> GSAEDKSKRDSIGLNAKEGQTNNGFVQNEDILETDLDPSSPAAGPQHNTVDILGPGEPDVKDVRPYAGMPKEVLFQFSGQARYRIPREVLFWLTVASVLLLIAATIAIIAISPKCLDWWQAGPMYQIYPRSFRDSNKDGDGDLKGIQDKLDYITTLNIKTVWITSFYKSSLKDFRHAVEDFQEIDPIFGTMKDFENLVAAIHDKGLKLIIDFIPNHTSDKHAWFQWSRNRTGKYTDYYIWHDCNYENGTTIPPNNWLSVYGNSSWHFDEVRKQCYFHQFMKEQPDLNFRNPDVQEEIKEIIQFWLSKGVDGFSFNALQYLLEAKHLRDEAQVNKTQIPDTVTHYSQLHHDFTTTQVGMHDIVRSFRQTMNQY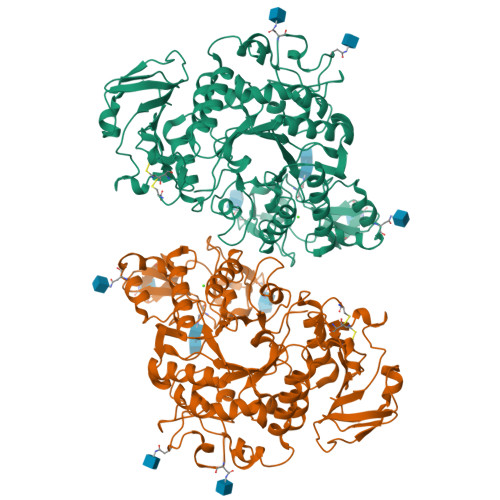SREPGRYRFMGTEAHGESITETMVYYGLPFIQEADFPFNSYLSKLDKPSGNSVSEVITSWLENMPEGKWPNWMTGGPDNVRLTSRLGEKYVNIMNMLVFTLPGTPITYYGEEIGMRNILAANLNENYDTGTLFSKSPMQWDNSSNAGFSEGNHTWLPTSSDYHTVNVDVQKTQPRSALKLYQELSLLHANELLLSRGWFCYLRNDNHSIMYTRELDGINKVFLMVLNFGESSLLNLKEMISNIPTRVRIRLSTSSAYSGREVDTHAVTLASGEGLILEYNTGNLLHRQTAFKDRCFVSNRACYSRVLNILYSLC> EEPPTVALTVPAAALLPDGALGESIVRGRRYLSDTPAQLPDFVGNGLACRHCHPGRDGEVGTEANAAPFVGVVGRFPQYSARHGRLITLEQRIGDCFERSLNGRALALDHPALIDMLAYMSWLSQGVPVGAVVAGHGIPTLTLEREPDGVHGEALYQARCLACHGADG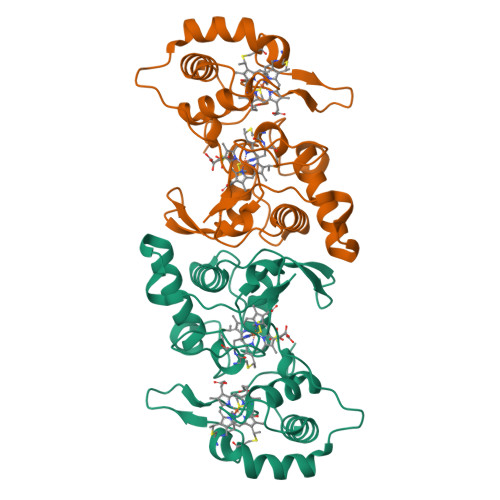SGTLDADGRYLFPPLWGPRSFNTGAGMNRQATAAGFIKHKMPLGADDSLSDEEAWDVAGFVLTHPRPLFQEPTGDASWSHPQFEK>MTNFDKISKMFWHYKDKIAQIKQDIVLPIKKADVNVRNLLSRHKRKINPKFGQLTNSNQQLFKIQNELTQLINDTKGDSLAYHWILNFIAKAVVHQAETEVRVKPESALPLGKLTLYLLVQFPELQELFMARLVKKCPFVIGFTCEIDTEKGRQNMGWKRNNENKWEDNTSYDERMGGILSLFAIITRLQLPQEFITTTSHPFPIALSWHILARICNTPLNLITNTHFVILGSWWDAAAVQFLQAYGNQASKLLILIGEELTSRMAEKKYVGAA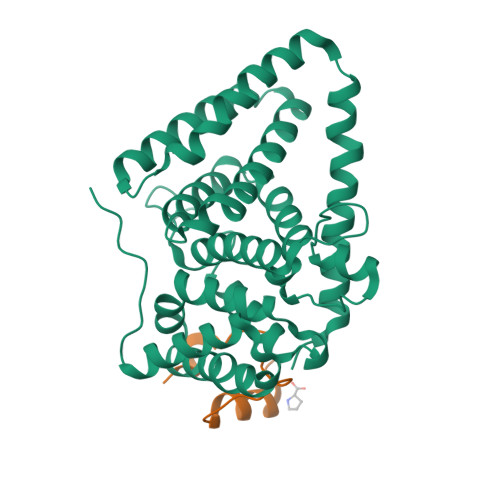RLRILLEAWQNNNMESFPEMSP[2x];>GPSGSELADLAEETLKIFRANKFELGLVPDIPPPPALVA[2x]>MRGSHHHHHHGSMDKNIIIGAMTALITPFKNGKVDEQSYARLIKRQIENGIDAVVPVGTTGESATLTHEEHRTCIEIAVETCKGTKVKVLAGAGSNATHEAVGLAKFAKEHGADGILSVAPFYNKPTQQGLYEHYKAIAQSVDIPVLLYNVPGRTGCEISTDTIIKLFRDCENIYGVKEASGNIDKCVDLLAHEPRMMLISGEDAINYPILSNGGKGVISVTSNLLPDMISALTHFALDENYKEAKKINDELYNINKILFCESNPIPIKTAMYLAGL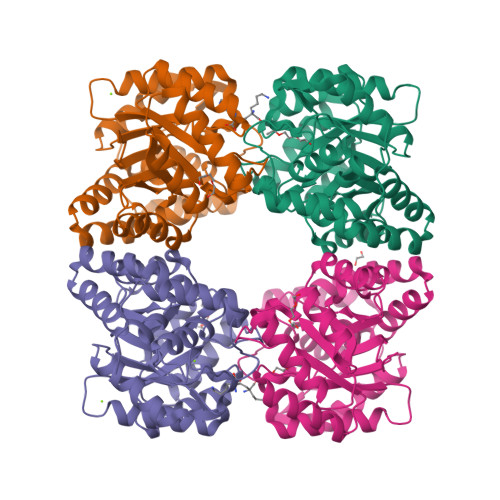IESLEFRLPLCSPSKENFAKIEEVMKKYKIKGF[4x]>[2x]SNAMSDIISIKDIDLAKKKVFIRCDFNVPQDDFLNITDDRRIRSAIPTIRYCLDNGCSVILASHLGRPKEISSKYSLEPVAKRLARLLDKEIVMAKDVIGEDAKTKAMNLKAGEILLLENLRFEKGETKNDENLAKELASMVQVYINDAFGVCHRAHSSVEAITKFFDEKHKGAGFLLQKEIDFASNLIKHPARPFVAVVGGSKVSGKLQALTNLLPKVDKLIIGGGMAFT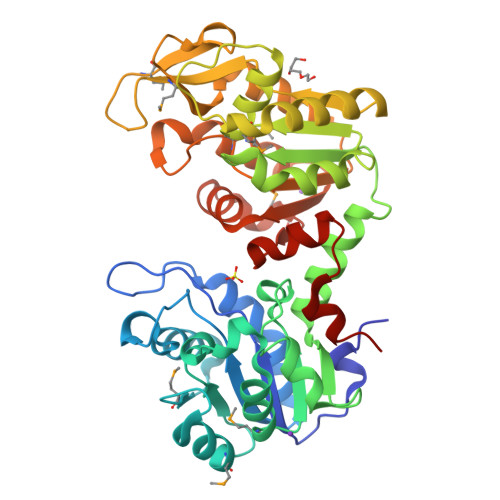FLKALGYDIGNSLLEEELLEEANKILTKGKNLGVKIYLPVDVVAAPACSQDVPMKFVPAQEIPNGWMGLDIGPASVRLFKEVISDAQTIWWNGPMGVFEIDKFSKGSIKMSHYISEGHATSVVGGGDTADVVARAGDADEMTFISTGGGASLELIEGKELPGVKALRSKENE>MHHHHHHLKNGMRPIHPG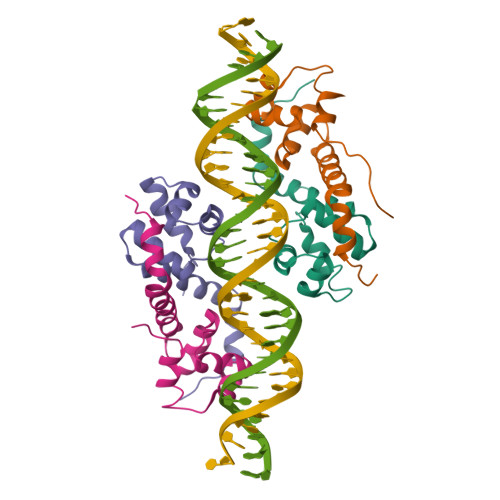EILREEFQKEMGFSAAALARALGVATPTVNNILRERGGVSADMALRLSICLDTTPEFWLNLQTAFDLRTAEQQHGDEIIGSVQRLVA[4x]>GPGSLTVYQGANATNYQQYKKKGVQFDDLLAINSDVMAWLTVKGTHIDYPIVQGENNLEYINKSVEGEYSLSGSVFLDYRNKVTFEDKYSLIYAHHMAGNVMFGELPNFRKKSFFNKHKEFSIETKTKQKLKINIFACIQTDAFDSLLFNPIDVDISSKNEFLNHIKQKSVQYREILTTNESRFVALS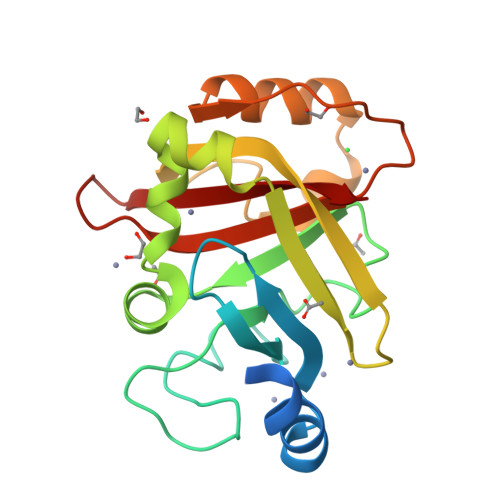TCEDMTTDGRIIVIGQIE[2x]MpPA14 (Marinomonas primoryensis PA14 domain) lectin is a domain of a 1.5-MDa adhesin responsible for a symbiotic bacterium-diatom interaction in Antarctica. Bioinformatic analyses indicated the presence of an ∼20-kDa domain near the C terminus of MpIBP that is a member of the PA14 family, which is a carbohydrate-binding lectin module widely distributed across several kingdoms of life. PA14 domains share a β-sandwich fold and the presence of two consecutive aspartate residues in a cis peptide linkage (DcisD). The DcisD motif coordinates a Ca2+ ion that is directly involved in binding polar vicinal hydroxyl groups of various carbohydrates.

With the C-3 hydroxyl in the axial position, allopyranose cannot bind MpPA14 via its cis vicinal 3,4-diol, as this would cause the saccharide ring to clash with residues of L11 (e.g., Gln156). Unexpectedly, the binding site of the lectin contained the furanose form of allose, with its 2,3-diol interacting with Ca1. The furanose rings lean toward L11, with their endocyclic oxygen interacting with the side chain amide group of Gln156, and the C-5 hydroxyl group extends out to hydrogen bond with the side chain hydroxyl of Ser130. At 30°C, approximately 92% of allose exists as pyranoses in solution, yet MpPA14 binding appears to be dependent on the rare presence of the allofuranose, which only makes up ∼8% of allose in solution, explaining the feeble affinity of this sugar for the lectin. Remarkably, the lectin can discern favorable conformations of these monosaccharides from their nonbinding anomers, even when the latter are much more prevalent in the equilibria (e.g., allofuranose as opposed to allopyranose).

> PKAQDDSTPDSLFAGLVGEYYGTNSQLNNISDFRALVDSKEADATFEAANISYGRGSSDVAKGTHLQEFLGSDASTLSTDPGDNTDGGIYLQGYVYLEAGTYNFKVTADDGYEITINGNPVATVDNNQSVYTVTHASFTISESGYQAIDMIWWDQGGDYVFQPTLSADGGSTYFVLDSAILSSTGETPYTTAQ> SASEEQVAQDTEEVFRSYVFYRHQQEQEAEGVAAPADPEMVTLPLQPSSTMGQVGRQLAIIGDDINRRYDSEFQTMLQHLQPTAENAYEYFTKIATSLFESGINWGRVVALLGFGYRLALHVYQHGLTGFLGQVTRFVVDFMLHHCIARWIAQRGGWVAALNLCNG;> EDIIRNIARHLAQWGDSMDRSW

Mitochondrial poration by pore-forming BCL-2 Effectors, BAK and BAX, initiates apoptosis. BAK is dormant in healthy cells. Its apo structure exhibits a stable globular conformation incapable of executing poration. Autoactivation is mechanistically similar to direct activation: binding of exposed BH3 of BAK or activators to the activation groove induces conformational changes in the electrostatic network at the bottom of this groove destabilizing helix α1 to initiate BAK unfolding.

We determined the crystal structure of the non-covalent W(3)W(5) BID BH3:BAK complex, which reveals the largest opening seen in BH3:BAK complexes induced by W(3) displacement of Y89 side chain at the center of the activation groove of BAK. Strikingly, the buried electrostatic network that stabilizes helix α1 in this complex is re-established as in apo BAK, involving two hydrogen bonds between α1 R42 and α2 N86 and α3 D90, and two hydrogen bonds between α2 E46 and α5 R137 (electron density shown in Supplementary Fig. 9b). Our structure reveals a mechanism for BAK inactivation that differs from previous complexes of BAK inactivated by rationally-designed BIM-like BH3 ligands that directly glue helix α127. The W(3)W(5) BID BH3-BAK structure bolsters the mechanistic link between the BH3 ligand binding-induced helix α1 stabilization and destabilization, and inactivation and activation of BAK, respectively. The wide opening of the hydrophobic groove in W(3)W5 BID BH3-BAK complex offers a novel strategy of inactivating BAK by blocking the activation groove while stabilizing helix α1 through indirect contacts. A caveat to this strategy is that an inactivator may activate BAK if it falls off and BAK reverts to a transient intermediary state resembling the BH3-activated conformation with a destabilized helix α1 electrostatic network. In contrast, the cavities in activated BAK BH3-BAK and inactivated W(3)W(5) BID BH3-BAK complexes are more modest in size (64–70 Å3) whereas activated M(3)W(5) BID BH3-BAK complex exhibits no cavity at the activation groove.>EPVAEPDIMATNRVVHV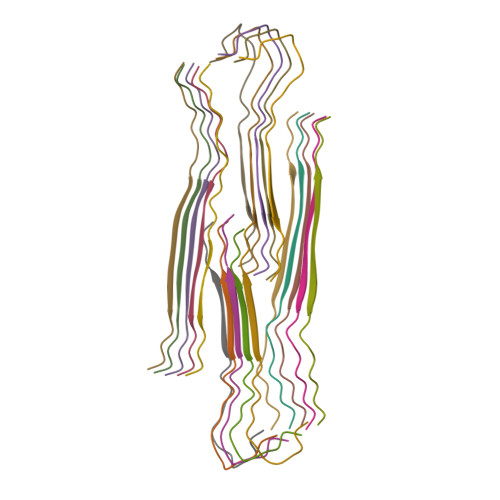ITNVLQ[20x]> GSSSKTLADNIETADLSASVPTRPAEPERKTLADYGGYPSALDAVKQKNDAAVAAYLENAGDSAMAENVRNEWLKSLGARRQWTLFAQEYAKLEPAGRAQEVECYADSSRNDYTRAAELVKNTGKLPSGCTKLLEQAAASGLLDGNDAWRRVRGLLAGRQTTDARNLAAALGSPFDGGTQGSREYALLNVIGKEARKSPNAAALLSEMESGLSLEQRSFAWGVLGHYQSQNLNVPAALDYYGKVADRRQLTDDQIEWYARAALRARRWDELASVISHMPEKLQKSPTWLYWLARSRAATGNTQEAEKLYKQAAATGRNFYAVLAGEELGRKIDTRNNVPDAGKNSVRRMAEDGAVKRALVLFQNSQSAGDAKMRRQAQAEWRFATRGFDEDKLLTAAQTAFDHGFYDMAVNSAERTDRKLNYTLRYISPFKDTVIRHAQNVNVDPAWVYGLIRQESRFVIGAQSRVGAQGLMQVMPATAREIAGKIGMDAAQLYTADGNIRMGTWYMADT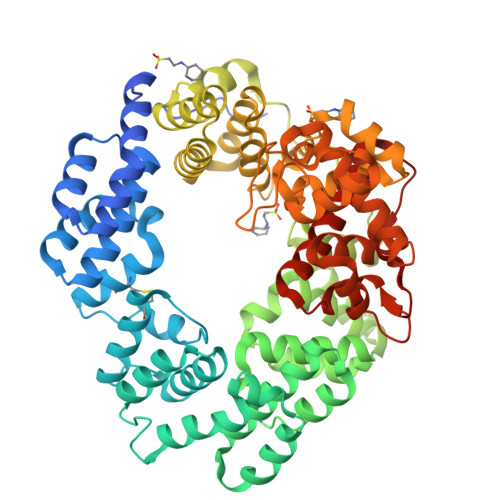KRRLQNNEVLATAGYNAGPGRARRWQADTPLEGAVYAETIPFSETRDYVKKVMANAAYYAALFGAPHIPLKQRMGIVPAR> GPLG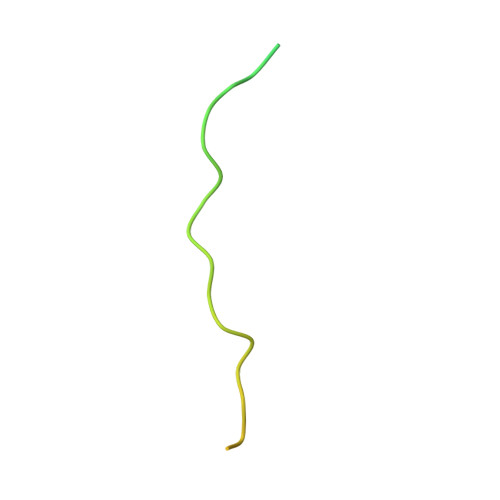SCYQNKLSISDHDSGVEDEDLSPRPSPNPHPVSQQTKRVHPLVPELSMVLDGSFLD>MEGIDHLADERNKAEFDVEDMKIVWAGSRHAFEVSDRIARLVASDPVFEKSNRARLSRKELFKSTLRKCAHAFKRIIELRLNEEEAGRLRHFIDQPAYVDLHWGMFVPAIKGQGTEEQQKKWLSLANKMQIIGCYAQTELGHGSNVQGLETTATLDPKTDEFVIHTPTQTASKWWPGGLGKVSTHAVVYARLITNGKDYGIHGFIVQLRSLEDHSPLPNITVGDIGTKMGNGAYNSMDNGFLMFDHVRIPRDQML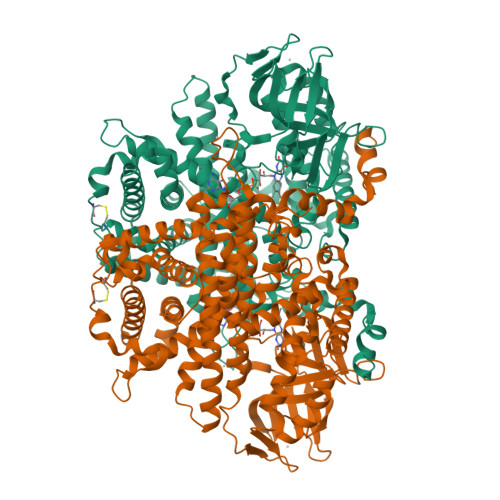MRLSKVTREGEYVPSDVPKQLVYGTMVYVRQTIVADASNALSRAVCIATRYSAVRRQFGAHNGGIETQVIDYKTQQNRLFPLLASAYAFRFVGEWLKWLYTDVTERLAASDFATLPEAHACTAGLKSLTTTATADGIEECRKLCGGHGYLWCSGLPELFAVYVPACTYEGDNVVLQLQVARFLMKTVAQLGSGKVPVGTTAYMGRAAHLLQCRSGVQKAEDWLNPDVVLEAFEARALRMAVTCAKNLSKFENQEQGFQELLADLVEAAIAHCQLIVVSKFIAKLEQDIGGKGVKKQLNNLCYIYALYLLHKHLGDFLSTNCITPKQASLANDQLRSLYTQVRPNAVALVDAFNYTDHYLNSVLGRYDGNVYPKLFEEALKDPLNDSVVPDGYQEYLRPVLQQQL[2x]>[2x]EFPEITEEMEKEIKNVFRNGNQDEVLSEAFRLTITRKDIQTLNHLNWLNDEIINFYMNMLMERSKEKGLPSVHAFNTFFFTKLKTAGYQAVKRWTKKV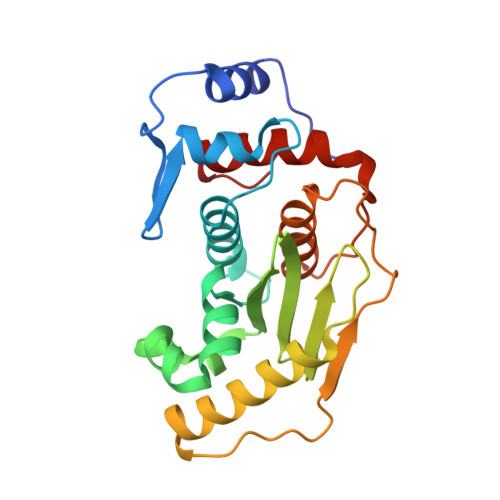DVFSVDILLVPIHLGVHWCLAVVDFRKKNITYYDSMGGINNEACRILLQYLKQESIDKKRKEFDTNGWQLFSKKSQIPQQMNGSDCGMFACKYADCITKDRPINFTQQHMPYFRKRMVWEILHRKLL> MASVDFKTYVDQACRAAEEFVNVYYTTMDKRRRLLSRLYMGTATLVWNGNAVSGQESLSEFFEMLPSSEFQISVVDCQPVHDEATPSQTTVLVVICGSVKFEGNKQRDFNQNFILTAQASPSNTVWKIASDCFRFQDWAS;> APPCKGSYFGTENLKSLVLHFLQQYYAIYDSGDRQGLLDAYHDGACCSLSIPFIPQNPARSSLAEYFKDSRNVKKLKDPTLRFRLLKHTRLNVVAFLNELPKTQHDVNSFVVDISAQTSTLLCFSVNGVFKEVDGKSRDSLRAFTRTFIAVPASNSGLC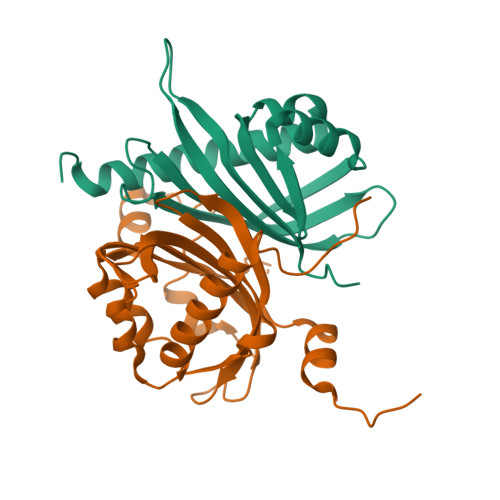IVNDELFVRNASSEEIQRAFAMPAPTPSSSPVPTLSPEQQEMLQAFSTQSGMNLEWSQKCLQDNNWDYTRSAQAFTHLKAKGEIPEVAFMK> MLTPTPDSSPRSTSSPSQSKNGSFTPRTANILKPLMSPPSREEIMAT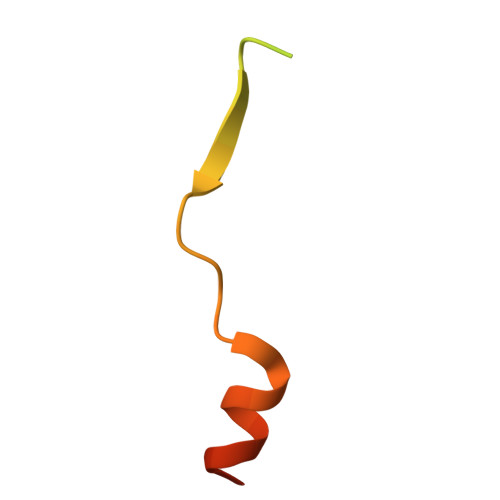LLDHD>[2x]AM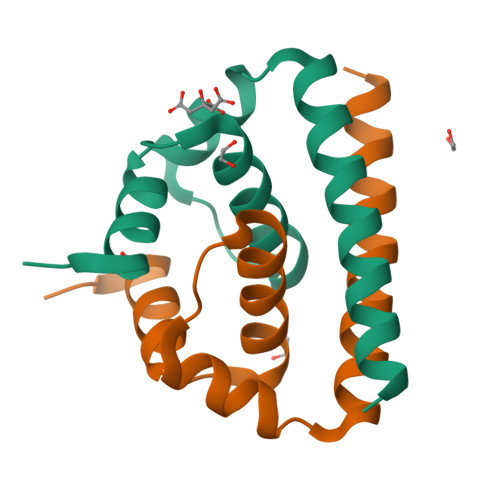ADIGSMTKKPGGPGKNRAINMLKRGLPRVFPLVGVKRVVMSLLDGRGPVRFVLALITFFKFTALAPTKALLGRWKAVEKSVAMKHLTSFKRELGTLIDAVNKRGRKQNKR> MAINFKGSPYLDRFDPSKDRTKVLFNPDRPLQQAELNEMQSIDQYYLKNLGDAIFKDGDKQSGLGFTLSEDNVLTVNPGYVYINGKIRYYDNDDSVKITGVGKETIGIKLTERIVTPDEDASLLDQTSGVPSYFSKGADRLEEKMSLTVNDPTSATIYTFMDGDLYIQSTNAEMDKINKVLAERTYDESGSYKVNGFELFSEGNAEDDDHVSVVVDAGKAYVKGFKVDKPVSTRISVPKSYDLGTAENESTIFNKSNNSISLANSPVKEIRRVTGQVLIEKERVTRGAQGDGQDFLSNNTAFEIVKVWTETSPGVTTKEYKQGEDFRLTDGQTIDWSPQGQEPSGGTSYYVSYKYNKRMEAGKDYEVTTQGEGLSKKWYINFTPSNGAKPIDQTVVLVDYTYYLARKDSVFINKYGDIAILPGEPNIMRLVTPPLNTDPENLQLGTVTVLPDSDEAVCISFAITRLSMEDLQKVKTRVDNLEYNQAVNALDDGAMEGQNPLTLRSVFSEGFISLDKADITHPDFGIVFSFEDAEATLAYTEAVNQPKIIPGDTTAHIWGRLISAPFTEERTIYQGQASETLNVNPYNIPNKQGVLKLTPSEDNWIDTENVTITEQKTKKVTMKRFWRHNESYYGETEHYLYSNLQ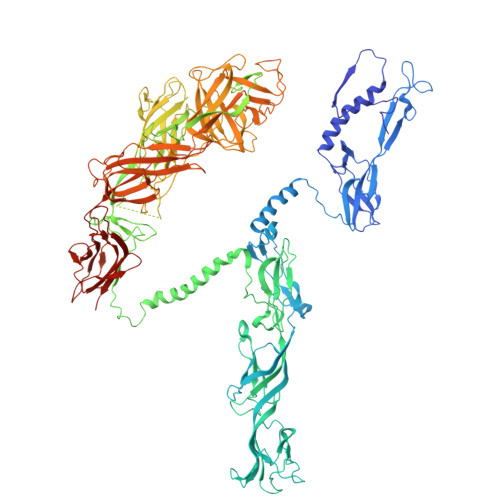LDAGQKWKGETYAYDREHGRTGTLLESGGQRTLEEMIEFIRIRDVSFEVKGLNPNDNNLYLLFDGVRCAITPATGYRKGSEDGTIMTDAKGTAKGKFTIPAGIRCGNREVTLKNANSTSATTYTAQGRKKTAQDIIIRTRVTVNLVDPLAQSFQYDENRTISSLGLYFASKGDKQSNVVIQIRGMGDQGYPNKTIYAETVMNADDIKVSNNASAETRVYFDDPMMAEGGKEYAIVIITENSDYTMWVGTRTKPKIDKPNEVISGNPYLQGVLFSSSNASTWTPHQNSDLKFGIYTSKFNETATIEFEPIKDVSADRIVLMSTYLTPERTGCTWEMKLILDDMASSTTFDQLKWEPIGNYQDLDVLGLARQVKLRATFESNRYISPLMSSSDLTFTTFLTELTGSYVGRAIDMTEAPYNTVRFSYEAFLPKGTKVVPKYSADDGKTWKTFTKSPTTTRANNEFTRYVIDEKVKSSGTNTKLQVRLDLSTENSFLRPRVRRLMVTTRDE> MERTELLKPRTLADLIRILHELFAGDEVNVEEVQAVLEAYESNPAEWALYAKFDQYRYTQNLVDQGNGKFNLMILCWGE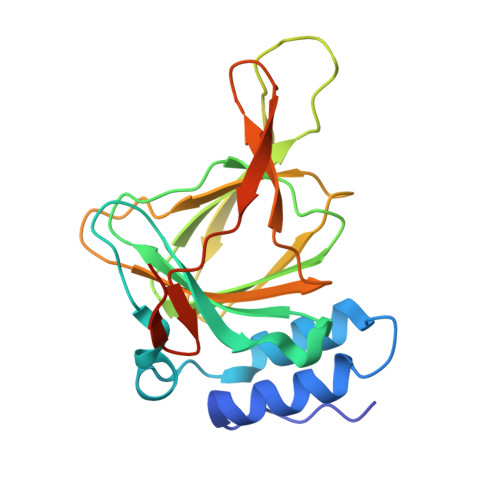GHGSSIHDHTDSHCFLKLLQGNLKETLFDWPDKKSNEMIKKSERTLRENQCAYINDSIGLHRVENVSHTEPAVSLHLYSPPFDTRHAFDQRTGHKNKVTMTFHSKFGIRTPFTTSGSLENN>[2x]MGSSHHHHHHSSGRENLYFQGMATAQPRGTPREQARLLKELADIQQLQRAHDSEPAATHSTSHGVSAQIVGGDIHRWRGFIAGPLGTPYEGGHFTLDIVIPPDYPYNPPKMK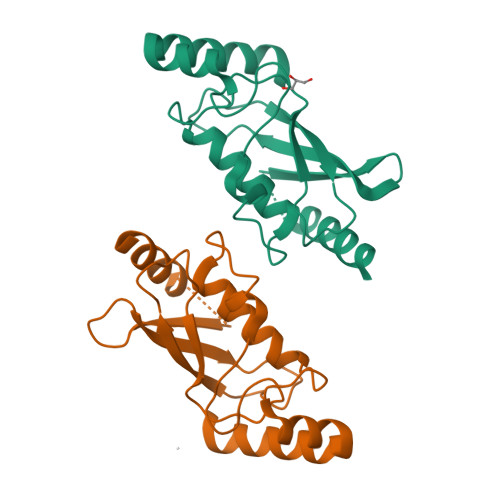FVTKIWHPNISSQTGAICLDILKHEWSPALTIRTALLSIQAMLADPVPTDPQDAEVAKMMIENHPLFVQTAKLWTETFAKE>[10x]MKGGAGVPDLPSLDASGVRLAIVASSWHGKICDALLDGARKVAAGCG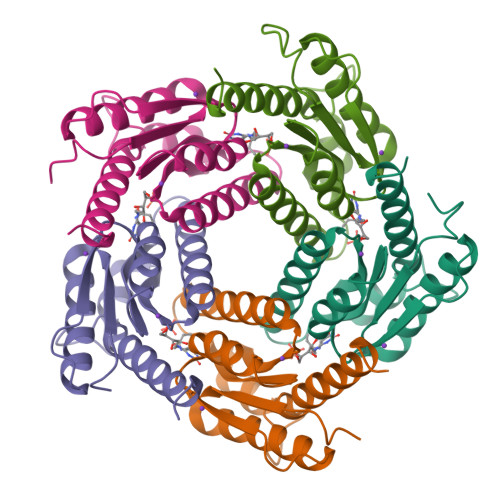LDDPTVVRVLGAIEIPVVAQELARNHDAVVALGVVIRGQTPHFDYVCDAVTQGLTRVSLDSSTPIANGVLTTNTEEQALDRAGLPTSAEDKGAQATVAALATALTLRELRAHS>GSDSPKPLPGPHLEPSCLSRGAHEKFSVEEYLVHALQGSVSSGQAHSLTSLAKTWAARGSRSREPSPKTEDNEGVLLTEKLKPVDYEYREEVHWATHQLRLGRGSFGEVHRMEDKQTGFQCAVKKVRLEVFRAEELMACAGLTSPRIVPLYGAVREGPWVNIFMELLEGGSLGQLVKEQGCL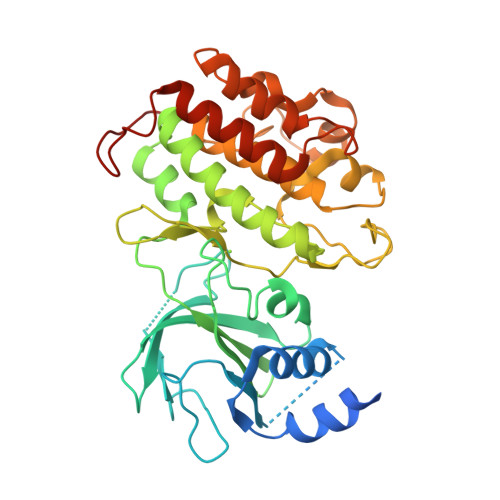PEDRALYYLGQALEGLEYLHSRRILHGDVKADNVLLSSDGSHAALCDFGHAVCLQPDGLGKSLLTGDYIPGTETHMAPEVVLGRSCDAKVDVWSSCCMMLHMLNGCHPWTQFFRGPLCLKIASEPPPVREIPPSCAPLTAQAIQEGLRKEPIHRVSAAELGGKVNRALQQVGGLKSPWRGEYKEPRGNS[4x]> QGMDFLTSTLLSGILYDGFKNGVAITTGFLKE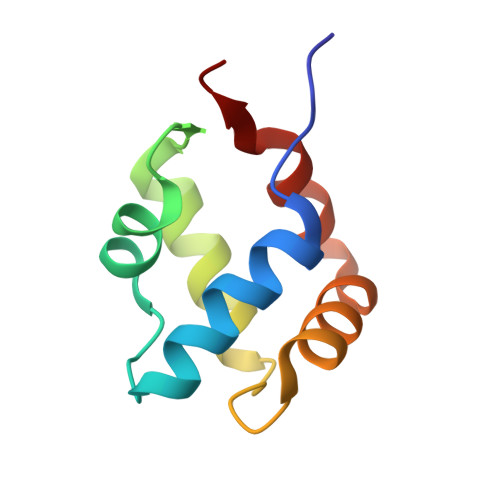KLHGWIVDDTLLETLAYKVNTLELKDYGEHVIERKLNESSEIQQILKLIQPEQ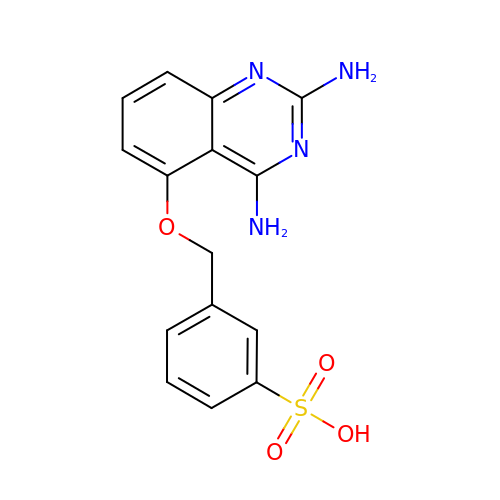3-{[(2,4-diaminoquinazolin-5-yl)oxy]methyl}benzenesulfonic acid | C15 H14 N4 O4 S | FEIMDUGCGJFTCE-UHFFFAOYSA-N Barrier-to-autointegration factor (BAF), encoded by the BANF1 gene, is an abundant and ubiquitously expressed metazoan protein that has multiple functions during the cell cycle. Through its ability to cross-bridge two double-stranded DNA (dsDNA), it favours chromosome compaction, participates in post-mitotic nuclear envelope reassembly and is essential for the repair of large nuclear ruptures. Phosphorylation of BAF by the vaccinia-related kinase 1 (VRK1) is a key regulator of BAF localization and function. Here, we demonstrate that VRK1 successively phosphorylates BAF on Ser4 and Thr3.

In order to obtain a detailed view of the structural consequences of BAF phosphorylation, we crystallized pBAF and solved its 3D structure at a resolution of 3.2 Å. While NMR revealed large chemical shift changes between BAF and pBAF, we did not observe any major structural changes due to phosphorylation in the crystal. Only helix 1 is significantly shortened in pBAF compared to BAF: it comprises residues 4–12 in BAF and is restricted to residues 7–11 in pBAF. And only residues Thr3, Ser4 and Gln5 have a Cα atom displaced by more than 2 Å after fitting the two structures. However, comparison of the dynamics of BAF and pBAF in solution by NMR revealed that the motions observed in BAF are strongly reduced in pBAF. As pThr3 and pSer4 are close to positively charged residues in helix α6 (Lys72, Arg75), electrostatic interactions between the phosphorylated side chains and helix α6 could explain the strong decrease in pBAF flexibility. We showed that the crystal structures of BAF and di-phosphorylated (pBAF) are similar. However, in solution, BAF exhibits large motions on both fast (picosecond to nanosecond) and slow (microsecond to milliesecond) timescales, which are not observed in pBAF. Thus, phosphorylation of Ser4 and Thr3 drastically reduces the conformational mobility of BAF. Consistently, phosphorylation causes a 5000-fold loss of affinity for dsDNA.

> TSQKHRDFVAEPMGEKPVGSLAGIGEVLGKKLEERGFDKAYVVLGQFLVLKKDEDLFREWLKDTAGANAKQSRDAFGALREWADAF>SNAAPQQINDIVHRTITPLIEQQKIPGMAVAVIYQGKPYYFTWGYADIAKKQPVTQQTLFELGSVSKTFTGVLGGDAIARGEIKLSDPATKYWPELTAKQWNGITLLHLATYTAGGLPLQVPDEVKSSSDLLRFYQNWQPAWAPGTQRLYANSSIGLFGALAVKPSGLSFEQAMQTRVFQPLKLNHTWINVPPPEEKNYA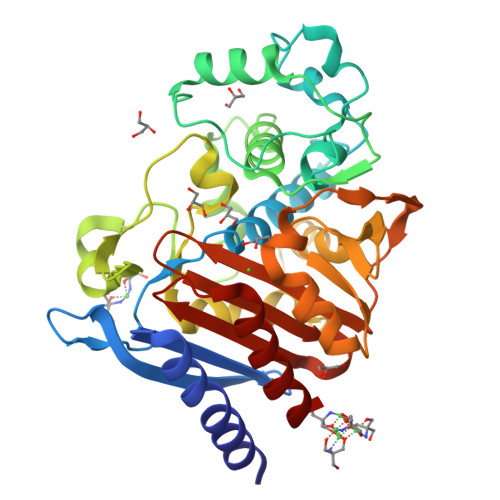WGYREGKAVHVSPGALDAEAYGVKSTIEDMARWVQSNLPPLDINEKTLQQGIQLAQSRYWQTGDMYQGLGWEMLDWPVNPDSIINGSDNKIALAARPVKAIKPPTPAVRASWVHKTGATGGFGSYVAFIPEKELGIVMLANKNYPNPARVAAACQILNALQ[2x]>[2x]GAPLSDSRVLWAPAEAHPLSPQGHPARLHRIVPRLRDVFGWGNLTCPICKGLFTAINLGLKKEPNVARVGSVAIKLCNLLKIAPPAVCQSIVHLFEDDMVEVWRRSVLSPSEACGLLLGSTCGHWDIFSSWNISLPTVPKPPPKPPSPPAPGAPVSRILFLTDLHWDHDYLEGTDPDCADPLCCRRGSGLPPASRPGAGYWGEYSKCDLPLRTLESLLSGLGPAGPFDMVYWTGDIPAHDVWHQTRQDQLRALTTVTALVRKFLGPVPVYPAVGNHESTPVNSFPPPFIEGNHSSRWLYEAMAKAWEPWLPAEALRTLRIGGFYALSPYPGLRLISLNMNFCSRENFWLLINSTDPAGQLQWLVGELQAAEDRGDKVHIIGHIPPGHCLKSWSWNYYRI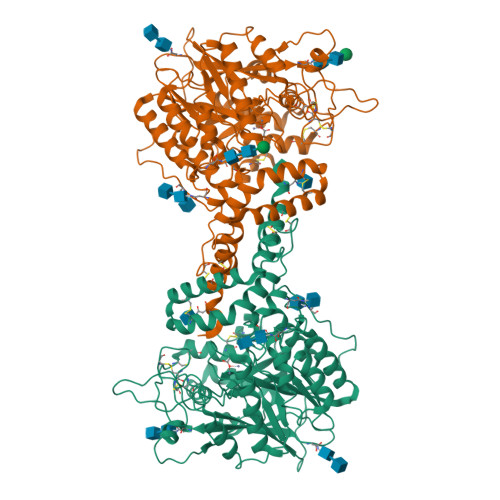VARYENTLAAQFFGHTHVDEFEVFYDEETLSRPLAVAFLAPSATTYIGLNPGYRVYQIDGNYSGSSHVVLDHETYILNLTQANIPGAIPHWQLLYRARETYGLPNTLPTAWHNLVYRMRGDMQLFQTFWFLYHKGHPPSEPCGTPCRLATLCAQLSARADSPALCRHLMPDGSLPEAQSLWPRPLFS> ENALLRYLLD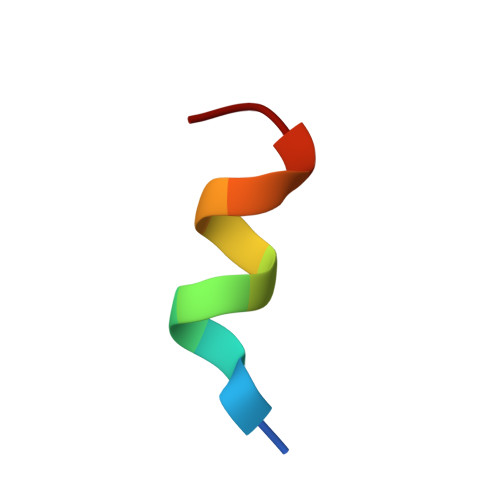KD In Gram-negative bacteria, Fe3+-siderophore complexes are recognised at the bacterial cell surface by highly selective outer-membrane TonB-dependent transporters (TBDTs). These transporters bind the Fe3+-siderophore complex and translocate it into the periplasm. The structures of pyoverdine, pyochelin, citrate and ferrichrome iron complexes bound to their respective transporters FpvA, FptA, FecA and FhuA showed that the ferric-siderophore complexes were bound inside the barrel adjacent to the plug domain, a position thought to be poised for translocation. Pseudomonas aeruginosa, a serious opportunistic pathogen, does not make enterobactin but does possess a TBTD outer-membrane protein PfeA, related to FepA, that binds and translocates Fe3+-enterobactin into the periplasm. PfeA has the same two domains (22-stranded β-barrel and N-terminal plug) common to the TBDTs.

Soaking of native crystals with Fe3+-enterobactin prior to data collection resulted in colour changes in the crystals. The data collected from such crystals revealed additional difference electron density that could unambiguously be modelled as a single Fe3+-enterobactin molecule. The ferric-siderophore is bound to PfeA by residues from loops L2, L3, L4, L7 and L11 on the extracellular surface, and is partly exposed to solvent. The side chain of Arg480 sits between rings I and II and makes electrostatic/cation-π interactions with ring II. The oxygen atoms O6 and O3 of catecholate III hydrogen bond to Ser479 and Gln482; O5 and O2 of the catecholate II hydrogen bond to the main chain nitrogen atoms of Arg480 and Gly325, whilst O4 of catecholate I hydrogen bonds to backbone nitrogen atom of Gln482. Comparison of the Fe3+-enterobactin complex structure with the apo-structure shows that L4 has undergone a large change (6.3 Å shift between Cα of G325) of conformation in order to interact with enterobactin molecule. The change in conformation of Glu327 of L4 results in the side-chain reaching further inside the pore to make a salt bridge with Arg100. In the Fe3+-enterobactin complex, the peptide bond at Pro28 (β-turn type II) flips resulting in the formation of an anti-parallel β-sheet rather than the α-helix and in disorder of the TonB box. We do see a correlation of movements between the binding site of the Fe3+-enterobactin molecule in the extracellular loops, the top of plug domain and the N-terminus. This suggests a route by which siderophore binding could be coupled to TonB engagement.

> AGQGDGSVIELGEQTVVATAQEETKQAPGVSIITAEDIAKRPPSNDLSQIIRTMPGVNLTGNSSSGQRGNNRQIDIRGMGPENTLILVDGKPVSSRNSVRYGWRGERDSRGDTNWVPADQVERIEVIRGPAAARYGNGAAGGVVNIITKQAGAETHGNLSVYSNFPQHKAEGASERMSFGLNGPLTENLSYRVYGNIAKTDSDDWDINAGHESNRTGKQAGTLPAGREGVRNKDIDGLLSWRLTPEQTLEFEAGFSRQGNIYTGDTQNTNSNNYVKQMLGHETNRMYRETYSVTHRGEWDFGSSLAYLQYEKTRNSRINEGLAGGTEGIFDPNNAGFYTATLRDLTAHGEVNLPLHLGYEQTLTLGSEWTEQKLDDPSSNTQNTEEGGSIPGLAGKNRSSSSSARIFSLFAEDNIELMPGTMLTPGLRWDHHDIVGDNWSPSLNLSHALTERVTLKAGIARAYKAPNLYQLNPDYLLYSRGQGCYGQSTSCYLRGNDGLKAETSVNKELGIEYSHDGLVAGLTYFRNDYKNKIESGLSPVDHASGGKGDYANAAIYQWENVPKAVVEGLEGTLTLPLADGLKWSNNLTYMLQSKNKETGDVLSVTPRYTLNSMLDWQATDDLSLQATVTWYGKQKPKKYDYHGDRVTGSANDQLSPYAIAGLGGTYRLSKNLSLGAGVDNLFDKRLFRAGNAQGVVGIDGAGAATYNEPGRTFYTSLTASF>SLLNVPAGKDLPEDIYVVIEIPANADPIKYEIDKESGALFVDRFMSTAMFYPCNYGYINHTLSLDGDPVNVLVPTPYPLQPGSVTRCRPVGVLKMTDEAGEDAKLVAVPHSKLSKEYDHIKDVNDLPELLKAQIAHF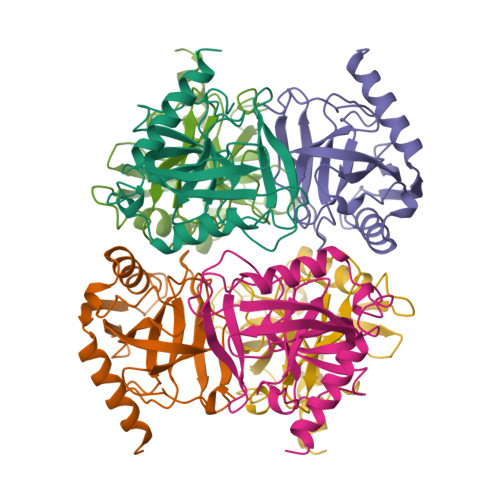FEHYKDLEKGKWVKVEGWENAEAAKAEIVASFERAKNK[2x]> MRVWVLAPHSLPPASFRPIFEARPPSSPTHSFHLLPTPIYLYITCTDAVDLYVCAVTSLLAEWTTTMF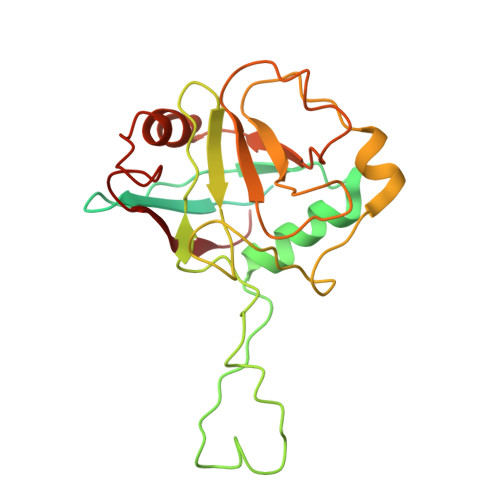ARSTIRWAAGAGHAFMDIAIGSQPPHRVTFELFTKRCPIASENFLKLCTGENVLPQVSSIDGIGEPSFRDQFLPQLTYRNTTVHRVCKGYLVQGGDIVSGQGTGQLSIYGESFDAPEEVKASKFDRMGLLGTAVSAPHLNGSQFFILTADKAPHLNGTCICFGRVVDGWTVVKAIEAIPLTAAGEPAERVVVVECGKL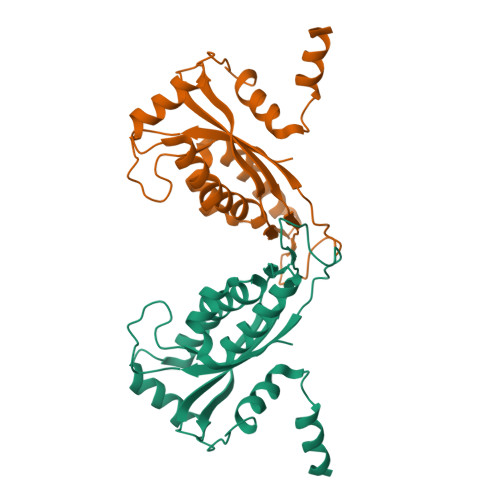> SIQSLKNKLWDESENPLIVVMRKITNKVGGFFAETESSRVYSQFKLMDPTFSNESFTRHLREYIVPEILEAYVKGDVKVLKKWFSEAPFNVYAAQQKIFKEQDVYADGRILDIRGVEIVSAKLLAPQDIPVLVVGCRAQEINLYRKKKTGEIAAGDEANILMSSYAMVFTRDPEQIDDDETEGWKILEFVRG> GPQRNGRAPEGKMDLIIMRGDKGFGFRLSGATHSAAEQTAQGQWVRNVD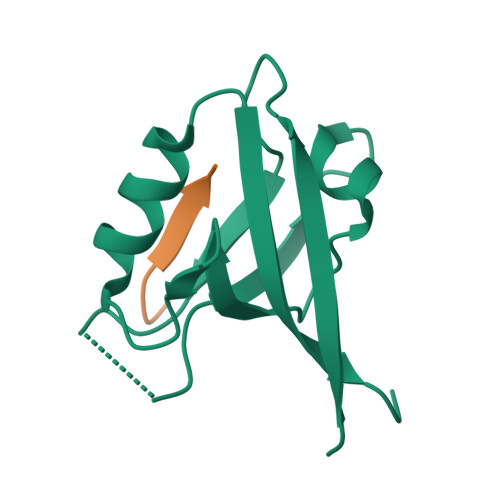PDGQAARAGLQAGDRLLELNGVDVSFWSHRKVVDEIKRSGDVVAFRIARRLSPGPD;> LPPPESESKV> KNNTLWTGPKPEANCIIEYGKQNPDSKLTLILVKNGGIVNGYVTLMGASDYVNTLFKNKNVSINVELYFDATGHILPDSSSLKTDLELKY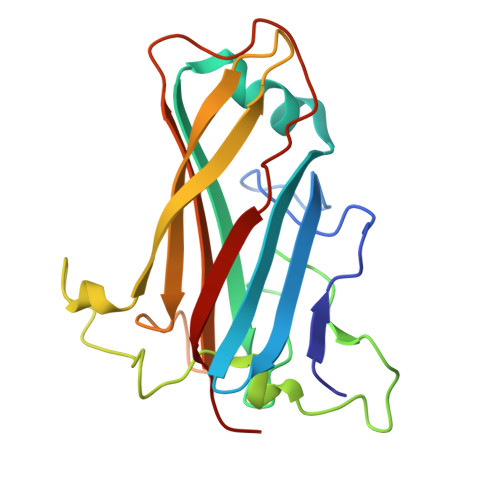KQTADFSARGFMPSTTAYPFVLPNAGTHNENYIFGQCYYKASDGALFPLEVTVMLNKRLPDSRTSYVMTFLWSLNAGLAPETTQATLITSPFTFSYIREDD>[4x]MARKYFVAANWKCNGTLESIKSLTNSFNNLDFDPSKLDVVVFPVSVHYDHTRKLLQSKFSTGIQNVSKFGNGSYTGEVSAEIAKDLNIEYVIIGHFERRKYFHETDEDV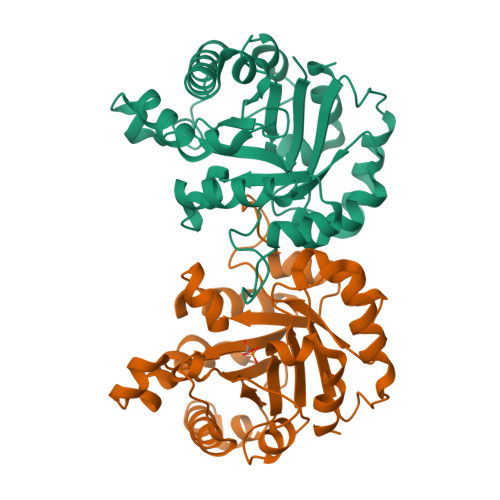REKLQASLKNNLKAVVCFGESLEQREQNKTIEVITKQVKAFVDLIDNFDNVILVYEPLWAIGTGKTATPEQAQLVHKEIRKIVKDTCGEKQANQIRILYGGSVNTENCSSLIQQEDIDGFLVGNASLKESFVDIIKSAM Kinetoplastids (such as Trypanosoma brucei), a group of evolutionarily divergent eukaryotes, have a unique set of kinetochore proteins that lack any significant homology to canonical kinetochore components. We previously identified KKT4 as a microtubule-binding kinetochore protein in T. brucei (throughout this manuscript we refer to KKT4 from Trypanosoma brucei unless stated otherwise) (Llauro et al., 2018). KKT4 directly binds to microtubules and maintains load-bearing attachments to both growing and shortening microtubule tips in vitro. KKT4 has the following predicted regions conserved among kinetoplastid species: an N-terminal α helix, a coiled-coil region and a block of basic residues in the microtubule-binding domain, and a BRCT domain at the C terminus.

To understand the function of the KKT4 BRCT domain, we solved its structure using X-ray crystallography. KKT4463–645 yielded crystals that diffracted to a resolution of 1.6 Å. The structure of KKT4463–645 revealed tandem BRCT domains. The N-terminal full domain (BRCT1) consists of a central four-stranded β sheet flanked by two α helices on one side of the sheet and one α helix on the opposite side. The smaller domain (BRCT2) consists of two α helices and three β strands, missing a β strand and an α helix in the C terminus. No electron density was observed for residues 463–473, 519–523, and 617–625, suggesting that these regions are flexible. Superposition of KKT4 BRCT1 with the N-terminal BRCT domain of H. sapiens BRCA1 showed a good structural match with an RMSD of 1.11 Å (for 65 Cα), suggesting that the KKT4 BRCT domain may bind phosphopeptides. In fact, we observed additional electron density in our structure, likely arising from a sulfate ion that may mimic a bound phosphate group. The sulfate ion is coordinated by three residues in the pocket, T494, S495, and K543, which correspond to the key residues known to interact with phosphopeptides in other BRCT domains (e.g., S1655, G1656, and K1702 in human BRCA1) (Williams et al., 2004). Furthermore, replacement of K543, located in the putative phosphopeptide-binding site in KKT4BRCT with alanine, decreased the binding affinity by roughly an order of magnitude.

> SMSGASSAVGGSTRSPSPVDPKRGAVQPRYFITTSLTEKERNSVMEAIQKLGQRAVLVDNKVDEILPLNTTHIVLRGPPRSVKALCGVVSSKWLVQPSYVFDSLGAGFWLDEEVEGGLRYFPPPLRCQRFLLTMPEGVVKTMLQRVVEFGGGEVVGTKRNGSSNDQDVVVVSSGDELLRFAISRD>[2x]MSVLISGASGYIAKHIVRVLLEQNYKVIGTVRSQDKADKLLKQYNNPNLSYEIVPEIANLDAFDDIFKKHG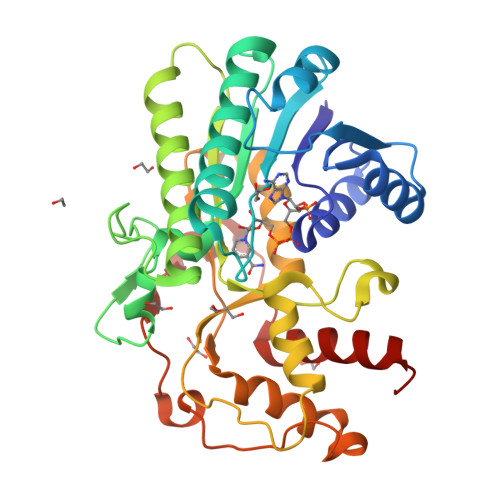KEIKYVIHAASPVNFGAKDLEKDLVIPAINGTKNMFEAIKKYAPDTVERVVMTASYASIMTPHRQNDPTLTLDEETWNPVTEENAYENVFTAYCASKTFAEKEAWKFVKENSDAVKFKLTTIHPSFVFGPQNFDEDVTKKLNETCEIINGLLHAPFDTKVEKTHFSQFIDVRDVAKTHVLGFQKDELINQRLLLCNGAFSQQDIVNVFNEDFPELKGQFPPEDKDTDLNKGVTGCKIDNEKTKKLLAFEFTPFHKTIHDTVYQILHKEGRV>[2x]MGK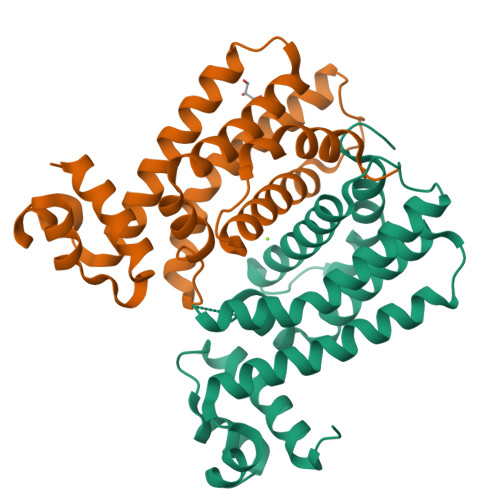KKGPKYDQIIDAAVQVIAEHGYHQAQVSKIAKAAGVADGTIYLYFNNKEDVLISLFQEKMGRFVDKIRSQMNEATDVEEKLKILVNMHFKQLAADHKLAIVTQLELRQSNTELALKINEVLKGYLNLLDELLMEGKEKGYFFQELDTRLARQMIFGTLDEVVTNWVMKDCKYDLTALVKPVHQLLLGGLRHR> MGHHHHHHSRGLVPRGSLSEKPNVKWEDVAGLEGAKEALKEAVILPVKFPHLFKGNRKPTSGILLYGPPGTGKSYLAKAVATEANSTFFSVSSSDLVSKWMGESEKLVKQLFAMARENKPSIIFI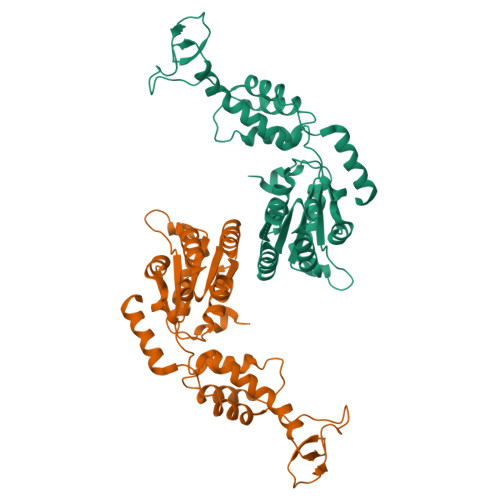DEVDALTGTRGEGESEASRRIKTELLVQMNGVGNDSQGVLVLGATNIPWQLDSAIRRRFERRIYIPLPDLAARTTMFEINVGDTPCVLTKEDYRTLGAMTEGYSGSDIAVVVKDALMQPIRKIQSATHFKDVSTEDDETRKLTPCSPGDDGAIEMSWTDIEADELKEPDLTIKDFLKAIKSTRPTVNEDDLLKQEQFTRDFGQEGN> MRNSKVVVVGTGFVGMSYAYAMVNQGTVEELVLLDIDKRKAEGEAMDLNHGLAFGPRKMSIKAGDYKDCKDAGLVVITAGVNQKEGETRIHLLKRNAEIIKTVVKNIMSSGFNGILLVASNPVDVLAYVAWKESGLHHSRV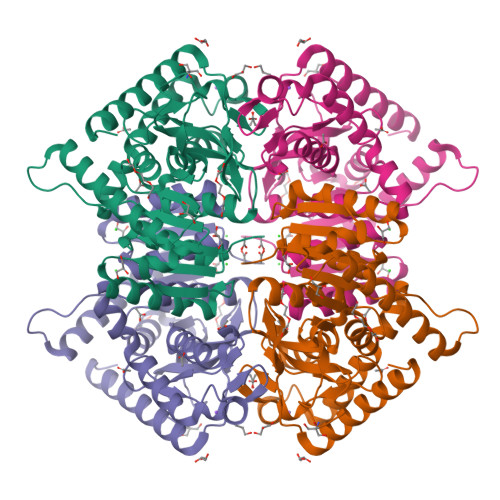IGSGTSLDTARLRYEISQYIHIDSRNVHAYILGEHGDSEFVCWSNANVGAKPIADVIDSMDEISFEDLEHIYLKVRDAAYEIISRKKATYYGIGMALVRITAAIFNNENRILPISVLNNGVYDCEDQVYIGLPAVLNKDGVHHIVKLKLNEKENSQLNNSANILRKNLDDMSY(1R,5S,6s)-3-[5-chloro-6-ethyl-2-(pyrimidin-5-ylsulfanyl)-7H-pyrrolo[2,3-d]pyrimidin-4-yl]-3-azabicyclo[3.1.0]hexan-6-amine | 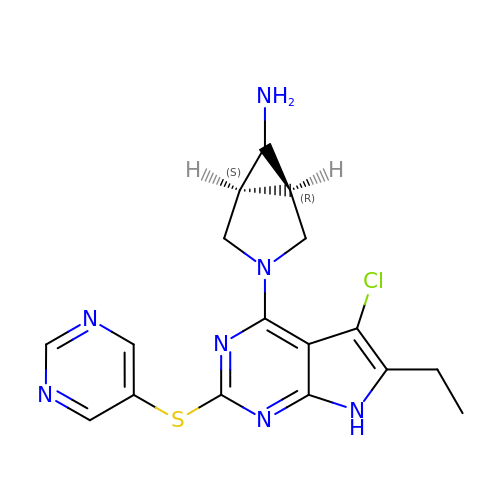C17 H18 Cl N7 S | OOKWYXHTSPTWDS-MSRIBSCDSA-N>[6x]MDREEMIARFAKFLREYVDDEGNEVYINRLKDLLTVTPKRSLAIDWAHLNSFDPELADELLNNPEEAIASAEDAIQIVLREPPLLVEREFKVHARFYNLPKTLLVKELGSEHINKLIQVEGIITRVSEVKPFVEKAVFVCRDCGNEMVRLQRPYENLVKPAKCDACGSRNIELDVDKSRFLNFQSFRLQDRPESLKGGQMPRFVDAILLDDLVDAALPGDRVLVTGVLRVILEQREKRPIFKKILE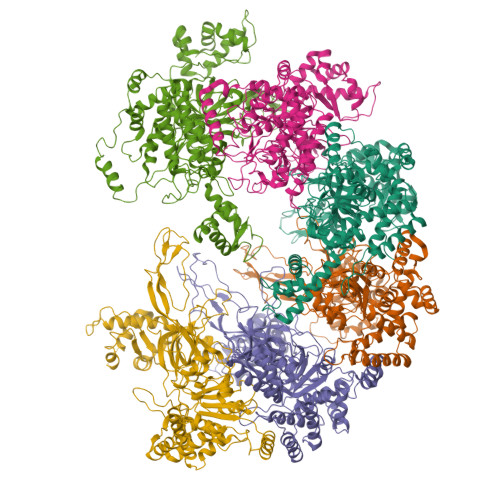VNHIEQLSKEIEELEISPEDEQKIRELAKRKDIVDAIVDSIAPAIWGHRIVKKGIALALFGGVQRTLPDGTKLRGESHVLLVGDPGVAKSQLLRYVANLAPRAIYTSGKSSSAAGLTAAAVRDEFTGSWVLEAGVLVLADGGFALIDEFDKMSDRDRSAIHEALEQQTISISKAGITATLNSRTTVIAAANPKFGRFNRHKSLPEQLDLPPTLLSRFDLIFLLLDEPDEKVDASIAEHILKVRRGEAEAVTPKIPYDLLKKYIAYARKNVHPVLSREAMEEIKRYYVKMRKGLRRGDEDGVQPIPITARQLEALIRLSEAHARMRLSETVTREDARAAIEIIEAMMKTIAVDEEGNLDVSILEVGKSSKKINKIEKLVDIIKSLESEGEFGAPEEKVIEAAKQAGIGTKADIEKLLNELKSDGRVYEPRAGFYRVI~{N}-[(4~{S},5~{R})-2-[2-(1~{H}-imidazol-4-yl)ethyl]-5-methyl-3-oxidanylidene-1,2-oxazolidin-4-yl]-2,3-bis(oxidanyl)benzamide 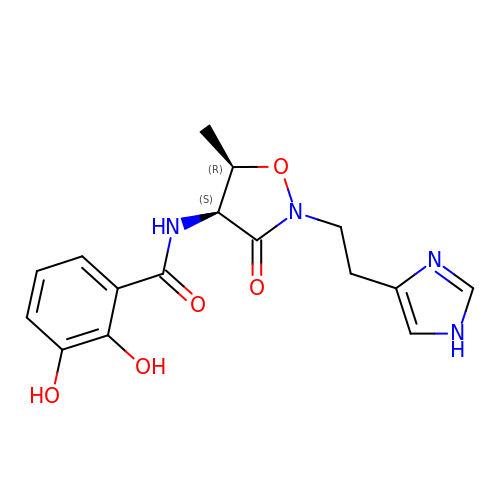| C16 H18 N4 O5 | YQXURFXJBIFMOA-RNCFNFMXSA-N> GGACAUUUAAUCGCGUGGAUA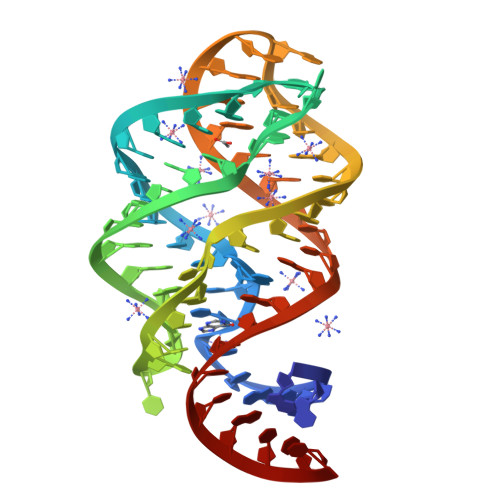UGGCACGCAAGUUUCUACCGGGCACCGUAAAUGUCCGACAAUGUCC>GELPEKSKLQEIYQELTQLKAAVGELPDQSKQQQIYQELTDLKTAFERLCRHCPKDWTFFQGNCYFMSNSQRNWHDSVTACQEVRAQLVVIKTAEEQNFLQLQTSRSNRFSWMGLSDLNQEGTWQWVDGSPLSPSF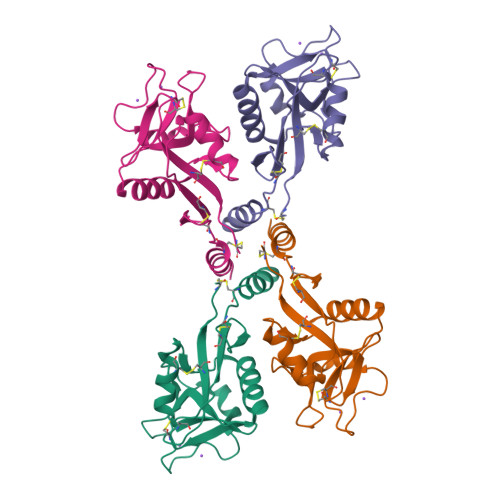QRYWNSGEPNNSGNEDCAEFSGSGWNDNRCDVDNYWICKKPAACFRDE[2x]>[2x]LE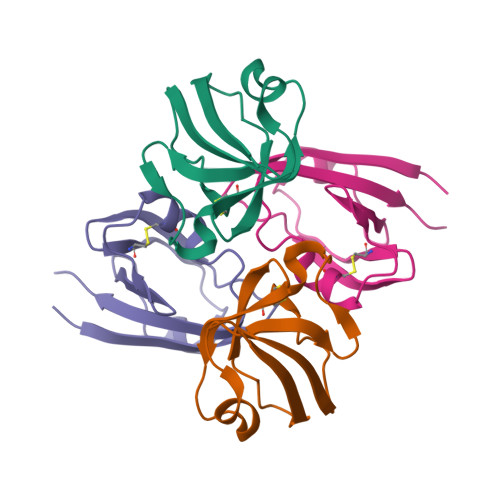KFNVDLMKKAGKELGLSLSPNEIGCTIADLIQGQYPEIDSKLQRGDIITKFNGDALEGLPFQVCYALFKGANGKVSMEVTRPKPAAAS5-(aminomethyl)-2-methyl-4-(4-methylphenyl)-6-(2-methylpropyl)pyridine-3-carboxic 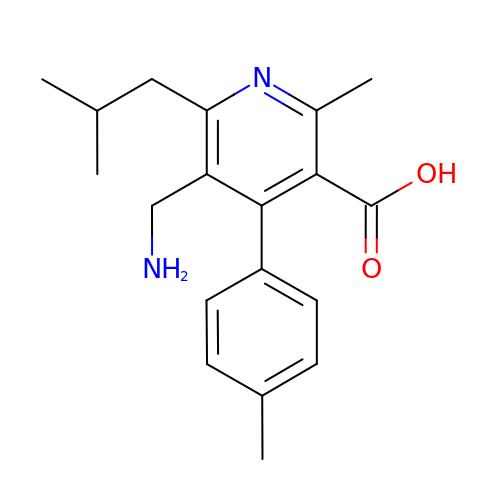acid | C19 H24 N2 O2 | NOAXOYPKZRNSHN-UHFFFAOYSA-N The biocatalytic reduction of the oxime moiety to the corresponding amine group has only recently been found to be a promiscuous activity of ene-reductases transforming α-oximo β-keto esters. By studying the crystal structures of enzyme oxime complexes, analyzing molecular dynamics simulations, and investigating biocatalytic cascades and possible intermediates, we obtained evidence that the reaction proceeds via an imine intermediate and not via the hydroxylamine intermediate. To gain more insight into the reaction pathway, we determined the crystal structures of the two enzymes OPR3 and XenA in complex with the oxime substrates 1a–c, either by co-crystallization or by soaking. All the crystal structures obtained had a high resolution (1.9–1.35 Å) and showed clear electron density features for the oximes.

To assess if the introduced amino acid exchanges affected the overall structure and the binding of the oxime, we also crystallized the tyrosine variants in complex with selected oxime substrates. The protomers in the crystal structures of the tyrosine variants are perfectly superimposable with the ones of the wild-type enzymes, confirming that the exchanges did not lead to major structural alterations. Interestingly, the binding mode of the oxime substrates also did not change in most of the structures. Testing the tyrosine variants for oxime reduction showed that the exchange of the non-canonical tyrosine Y370 to phenylalanine in OPR3 led to significantly decreased product formation compared to the wild type (OPR3_Y370F). This is true for the transformation leading to pyrazine 3a and the cascade with the alcohol dehydrogenase ADH-A leading to the amino alcohol 4a. In comparison to the wild type, the non-canonical tyrosine variant Y370F of OPR3 showed a 4-fold decrease in both kred and Kd in the reductive half-reaction and a 3- and 2-fold decrease in kox and Kd in the oxidative half-reaction. It is clear that Y370 plays some role in the binding and in the reactivity with reduced nicotinamide adenine dinucleotide phosphate (NADPH) as well as with the oxime. The effect of the Y370F mutation on the oxidative half-reaction is a clear indication that this residue has a role in the catalytic mechanism.

>[2x]MASSAQDGNNPLFSPYKMGKFNLSHRVVLAPMTRCRALNNIPQAALGEYYEQRATAGGFLITEGTMISPTSAGFPHVPGIFTKEQVREWKKIVDVVHAKGAVIFCQLWHVGRASHEVYQPAGAAPISSTEKPISNRWRILMPDGTHGIYPKPRAIGTYEISQVVEDYRRSALNAIEAGFDGIEIHGAHGYLIDQFLKDGINDRTDEYGGSLANRCKFITQVVQAVVSAIGADRVGVRVSPAIDHLDAMDSNPLSLGLAVVERLNKIQLHSGSKLAYLHVTQPRYVAYGQTEAGRLGSEEEEARLMRTLRNAYQGTFICSGGYTRELGIEAVAQGDADLVSYGRLFISNPDLVMRIKLNAPLNKYNRKTFFTQDPVVGYTDYPFLQGNGSNGPLSRLLEHHHHHH> NGYTYEDYQDTAKWLLSHTE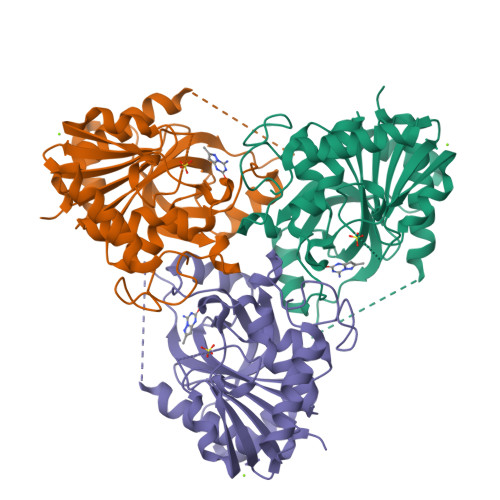QRPQVAVICGSGLGGLVNKLTQAQTFDYSEIPNFPESTVPGHAGRLVFGILNGRACVMMQGRFHMYEGYPFWKVTFPVRVFRLLGVETLVVTNAAGGLNPNFEVGDIMLIRDHINLPGFSGENPLRGPNEERFGVRFPAMSDAYDRDMRQKAHSTWKQMGEQRELQEGTYVMLGGPNFETVAECRLLRNLGADAVGMSTVPEVIVARHCGLRVFGFSLITNKVIMDYESQGKANHEEVLEAGKQAAQKLEQFVSLLMASIPV> 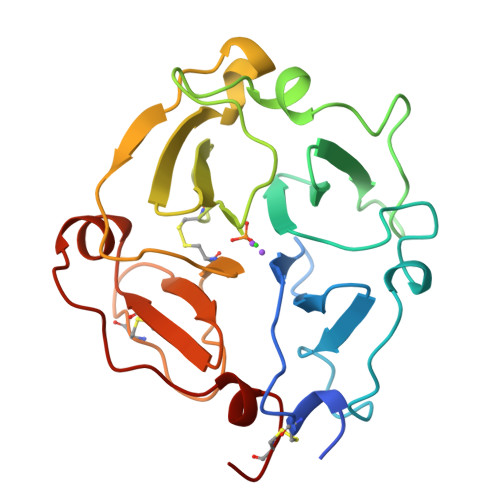HRNSTQHGHESTRCDPDLVLSAMVSDNHGATYVFSGSHYWRLDTNRDGWHSWPIAHQWPQGPSTVDAAFSWEDKLYLIQDTKVYVFLTKGGYTLVNGYPKRLEKELGSPPVISLEAVDAAFVCPGSSRLHIMAGRRLWWLDLKSGAQATWTELPWPHEKVDGALCMEKPLGPNSCSTSGPNLYLIHGPNLYCYRHVDKLNAAKNLPQPQRVSRLLGCTH> MGSSHHHHHHGSNQLTAYTLRLGDNCLVLSQRLGEWCGHAPELEIDLALANIG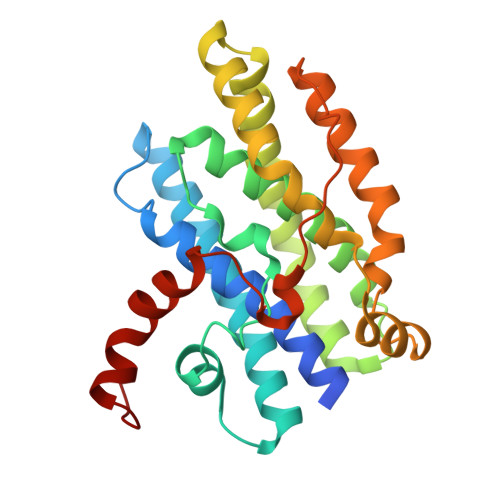LDLLGQARNFLSYAAELAGEGDEDTLAFTRDERQFSNLLLVEQPNGNFADTIARQYFIDAWHVALFTRLMESRDPQLAAISAKAIKEARYHLRFSRGWLERLGNGTDVSGQKMQQAINKLWRFTAELFDADEIDIALSEEGIAVDPRTLRAAWEAEVFAGINEATLNVPQEQAYRTGGKKGLHTEHLGPMLAEMQYLQRVLPGQQW>[4x]SMPEQSNDYRVVVFG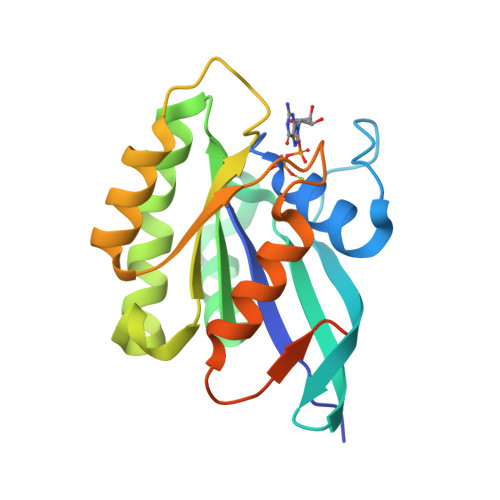AGGVGKSSLVLRFVKGTFRDTYIPTIEDTYRQVISCDKSVCTLQITDTTGSHQFPAMQRLSISKGHAFILVFSVTSKQSLEELGPIYKLIVQIKGSVEDIPVMLVGNKCDETQREVDTREAQAVAQEWKCAFMETSAKMNYNVKELFQELLTLETRRNMSLNIDGKRSGKQKRTDRVKGKCTLM> GNLAGAVEFNDVKTLLREWITTISDPMEEDILQVVKYCTDLIEEKDLEKLDLVIKYMKRLMQQSVESVWNMAFDFILDNVQVVLQQTY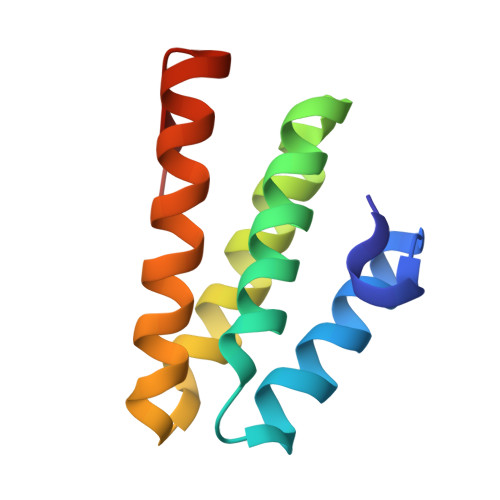GSTLKVT> MYMKKLVFGGMLIVSAASLVGCMSQIGSSVRQAVSDNQSAQTLVEWENSEANPEALFANWRHEFMVDSSKRESMKTELCKELQALPAQDLTLFENEIRDENNRALVSGCKEELLAQVDEHFDEQRESMSVPGHALKAVQSRNSFRFPDNTQKRDMSNGYMAVRGDVARKEVVLTFDDGPHGLYTDAILRALKEVNAKAMFFATGKSVRTNPEALKRVAADGHVIGSHSITHACLGTSVACYKQMGNRNLTFDEAAAEVRGGHQAVFDVLGWVDPVFRFXYGETSKDLKAFLKTKSTGEFAWNIESDDWRTQSNEQLLARVLANVESQGRGIV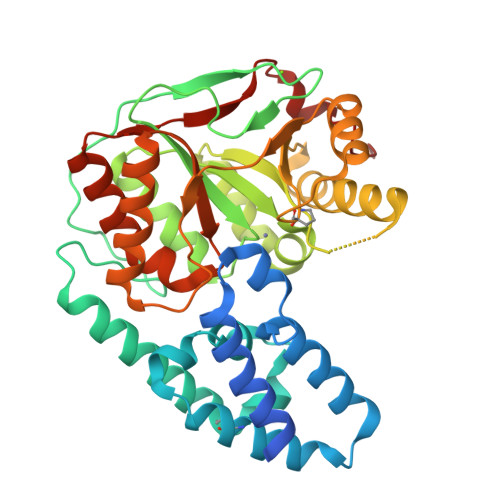LFHDIQRRTAEIMPQFLRELYNRGYSVVLLTAADPSAKYNSKLVKRKQQLP> MKKIITIVAMLLAMQGIAIAAGKIPTTTMGGKDFTFKPSTNVSVSYFTTNGATSTAGTVNTDYAVNTKNSSGNRVFTST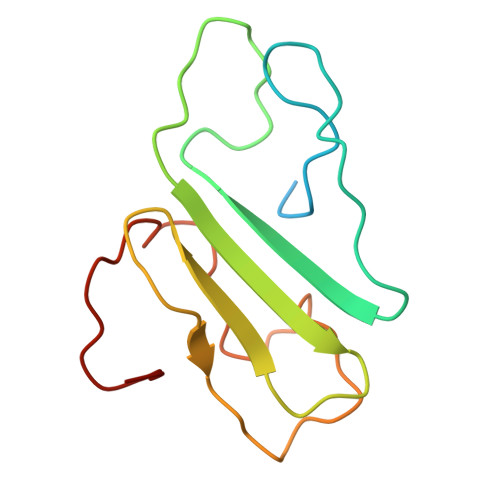NNTSNIWYIENDAWKGKAVSDSDVTALGTGDVGKSDFSGTEWKSQ>CCAIICCUII[4x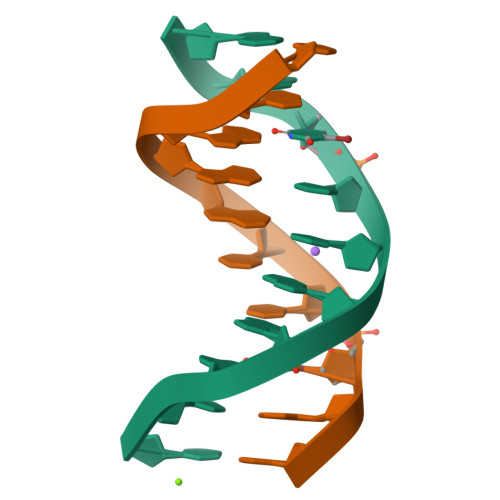]3'-DESAMINO-3'-(3-CYANO-4-MORPHOLINYL)-DOXORUBICIN 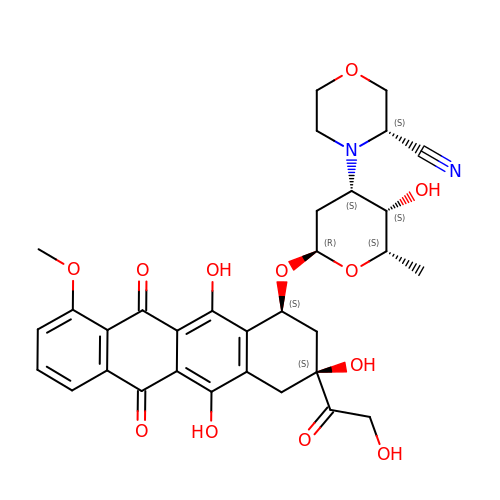| C32 H34 N2 O12 | YIMDLWDNDGKDTJ-USRAFFTGSA-N> DNPGTAPLDTFMTLSESLTGKKGLSRVIGERLLQALQKGSFKTADSLPQLAGALASGSLTPEQESLALTILEAWYLGIVDNVVITYEEALMFGVVS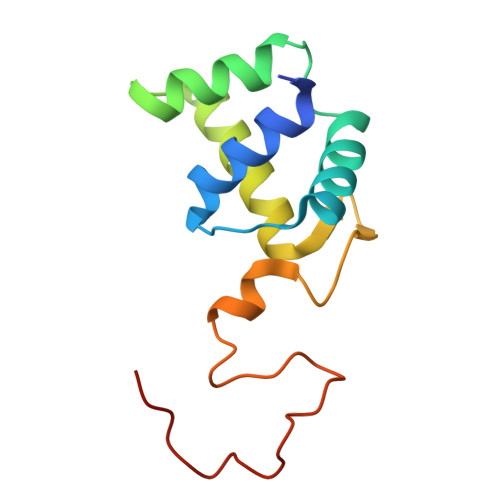DTLVIRSYCPNKPGFWADKPIERQA P2X receptors are the family of cation channels activated by extracellular ATP and are widely expressed in the mammalian nervous, respiratory, reproductive, and immune systems. There are seven subtypes (P2X1-P2X7) in the family, each of which plays distinct roles in physiological and pathophysiological functions via homo- or heterotrimerization. In this work, we determined the cryogenic electron microscopy (cryo-EM) structures of the panda P2X7 (pdP2X7) receptor in complex with PPADS and PPNDS. The overall structures are similar and show the trimeric architecture of P2X receptors, consisting of the extracellular domain and two transmembrane (TM) helices, with each protomer resembling the dolphin shape, consistent with the previously reported P2X structures (Sheng and Hattori, 2022).

The structures of pdP2X7 in the presence of PPNDS and PPADS were determined at 3.3 Å and 3.6 Å, respectively. More importantly, we identified the residual EM densities at the agonist binding site that fit into the shape of PPNDS and PPADS. It should be noted that while the pyridoxal phosphate groups in PPNDS and PPADS are shared, the naphthylazo group of PPNDS is significantly bulkier than the azophenyl group of PPADS. The phosphate group of PPNDS and PPADS interacts directly with the side chain of Arg294 and possibly also with Lys145, possibly via a water molecule. Interestingly, despite the structural differences between PPNDS and PPADS, the two common sulfonic acid groups form hydrogen bonds with the side chains of the same residues in the receptor, Lys66 and Gln143. Finally, to verify the binding mode of the pyridoxal phosphate derivatives, we performed molecular dynamics (MD) simulations of the higher-resolution PPNDS-bound structure embedded in lipids. The overall structures were stable during the simulations, and PPNDS remained stably bound to the receptor. In the PPNDS-bound structure, while we observed motion of the head domain similar to that in the ATP-bound structure, there was only a small structural change in the left flipper domain. Consequently, there was no structural change in the lower body domain or associated gating motion of the TM domain. Comparison with the previously reported apo- (closed) and ATP-bound (open) structures showed that, in contrast to ATP binding, the binding of PPNDS and PPADS does not induce the downward motion of the left flipper, which is essential for channel activation.

>[3x]GSSTNYGTIKWIFHALVFSYISFALISDKRYQKKEPLISSVHTKVKGIAEVKAEILENGMKKMVSGVFDTADYTFPLQGNSFFVMTNFIKTEGQQQGLCPDFPTARTICSSDRGCKKGRMDPQSKGIQTGRCVVYKERLKTCEVSAWCPIEEVKDAPRPALLNSAENFTVLIKNNIDFPGHNYTTRNILPGVNITCTFHKTQNPQCPIFRLGDIFQETGDSFSDVAIQGGIMGIEIYWDCNLDGWFHHCRPKYSFRRLDDKTTSESLYPGYNFRYAKYYKENNVEKRTLIKVFGIRFDILVFGTGGKFNVIQLAVYIGSVISYFGLATVFIDILINTYSASS N-{N-[4-(acetylamino)-3-chloro-5-methylbenzyl]carbamimidoyl}-3-(4-methoxyphenyl)-5-methyl-1,2-thiazole-4-carboxamide 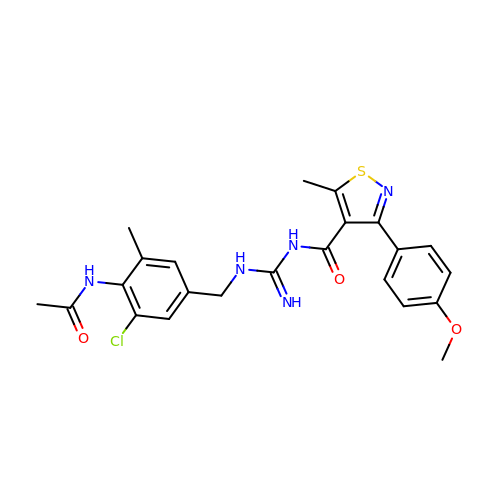| C23 H24 Cl N5 O3 S | MQPJKTGBSCCWTI-UHFFFAOYSA-N>[15x]MNSGLSRLGIALLAAMFAPALLAADLEKLDVAALPGDRVELKLQFDEPVAAPRGYTIEQPARIALDLPGVQNKLGTKNRELSVGNTRSVTVVEAKDRTRLIINLTALSSYTTRVEGNNLFVVVGNSPHHHHHHHHAGASVASAAPVKASPAPASYAQPIKPKPYVPAGRAIRNIDFQRGEKGEGNVVIDLSDPTLSPDIQEQGGKIRLDFAKTQLPDALRVRLDVKDFATPVQFVNASAQSDRT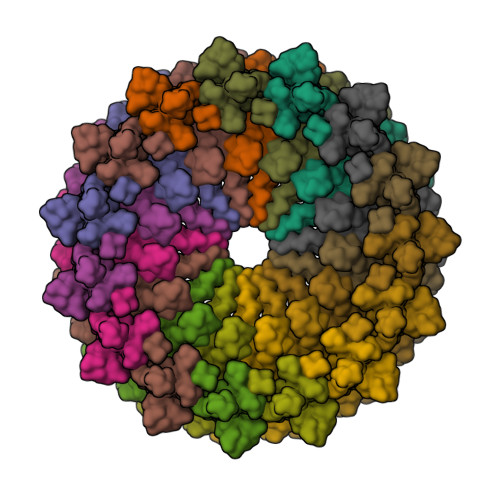SITIEPSGLYDYLVYQTDNRLTVSIKPMTTEDAERRKKDNFAYTGEKLSLNFQDIDVRSVLQLIADFTDLNLVASDTVQGNITLRLQNVPWDQALDLVLKTKGLDKRKLGNVLLVAPADEIAARERQELEAQKQIAELAPLRRELIQVNYAKAADIAKLFQSVTSDGGQEGKEGGRGSITVDDRTNSIIAYQPQERLDELRRIVSQLDIPVRQVMIEARIVEANVGYDKSLGVRWGGAYHKGNWSGYGKDGNIGIKDEDGMNCGPIAGSCTFPTTGTSKSPSPFVDLGAKDATSGIGIGFITDNIILDLQLSAMEKTGNGEIVSQPKVVTSDKETAKILKGSEVPYQEASSSGATSTSFKEAALSLEVTPQITPDNRIIVEVKVTKDAPDYQNMLNGVPPINKNEVNAKILVNDGETIVIGGVFSNEQSKSVEKVPFLGELPYLGRLFRRDTVTDRKNELLVFLTPRIMNNQAIAIGRGHHHHHHHH>MERHVPEPTHTLEGWHVLHDFRLLDFARWFSAPLEAREDAWEELKGLVREWRELEEAGQGSYGIYQVVGHKADLLFLNLRPGLDPLLEAEARLSRSAFARYLGRSYSFYSVVELGSQEKPLDPESPYVKPRLTPRVPKSGYVCFYPMNKRRQGQDNWYMLPAKERASLMKAHGETGRKYQGEVMQVISGAQGLDDWEWGVDLFSEDPVQFK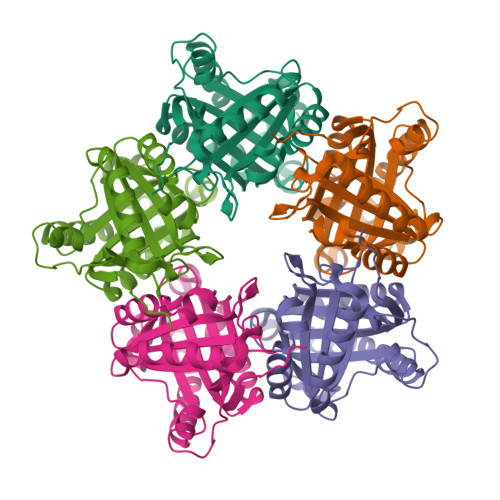KIVYEMRFDEVSARYGEFGPFFVGKYLDEEALRAFLGL[5x]> LEDVVVQAPTQVPGFLGDSVTLPCYLQVPNMEVTHVSQLTWARHGESGSMAVFHQTQGPSYSESKRLEFVAARLGAELRNASLRMFGLRVEDEGNYTCLFVTFPQGSRSVDIWLRVLAKPQNTAEVQKVQLTGEPVPMARCVSTGGRPPAQITWHSDLGGMPNTSQVPGFLSG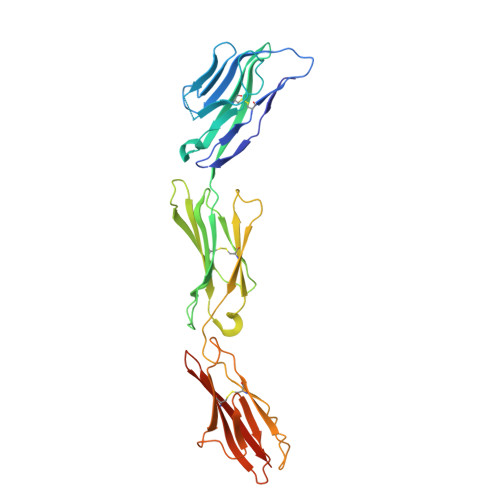TVTVTSLWILVPSSQVDGKNVTCKVEHESFEKPQLLTVNLTVYYPPEVSISGYDNNWYLGQNEATLTCDARSNPEPTGYNWSTTMGPLPPFAVAQGAQLLIRPVDKPINTTLICNVTNALGARQAELTVQVKEGPPTSHHHHHH>MLESKLKAPVFTATTQGDHYGEFVLEPLERGFGVTLGNPLRRILLSSIPGTAVTSVYIEDVLHEFSTIPGVKEDVVEIILNLKELVVRFLDPKMASTTLILRAEGPKEVRAGDFTPSADVEIMNPDLHIATLEEGGKLYMEVRVDRGVGYVPAERHGIKDRINAIPVDAIFSPVRRVAFQVEDTRLGQRTDLDKLTLRIWTDGSVTPLEALNQAVAILKEHLNYFANPEASLLPTPEVSKGEKRESAEEDLDLPLEELGLSTRVLHSLKEEGIESVRALLALNLKDLRNIPGIGERSLEEIRQALAKKGFTLKE[4x];>MEIKRFGRIREVIPLPPLTEIQVESYKKALQADVPPEKRENVGIQAAFKETFPIEEGDKGKGGLVLDFLEYRIGDPPFSQDECREKDLTYQAPLYARLQLIHKDTGLIKEDEVFLGHLPLMTEDGSFIINGADRVIVSQIHRSPGVYFTPDPARPGRYIASIIPLPKRGPWIDLEVEASGVVTMKVNKRKFPLVLLLRVLGYDQETLVRELSAYGDLVQGLLDEAVLAMRPEEAMVRLFTLLRPGDPPKKDKALAYLFGLLADPKRYDLGEAGRYKAEEKLGVGLSGRTLVRFEDGEFKDEVFLPTLRYLFALTAGVPGHEVDDIDHLGNRRIRTVGELMADQFRVGLARLARGVRERMVMGSPDTLTPAKLVNSRPLEAALREFFSRSQLSQFKDETNPLSSLRHKRRISALGPGGLTRERAGFDVRDVHRTHYGRICPVETPEGANIGLITSLAAYARVDALGFIRTPYRRVKNGVVTEEVVYMTASEEDRYTIAQANTPLEGDRIATDRVVARRRGEPVIVAPEEVEFMDVSPKQVFSLNTNLIPFLEHDDANRALMGSNMQTQAVPLIRAQAPVVMTGLEERVVRDSLAALYAEEDGEVVKVDGTRIAVRYEDGRLVEHPLRRYARSNQGTAFDQRPRVRVGQRVKKGDLLADGPASEEGFLALGQNVLVAIMPFDGYNFEDAIVISEELLKRDFYTSIHIERYEIEARDTKLGPERITRDIPHLSEAALRDLDEEGIVRIGAEVKPGDILVGRTSFKGEQEPSPEERLLRSIFGEKARDVKDTSLRVPPGEGGIVVGRLRLRRGDPGVELKPGVREVVRVFVAQKRKLQVGDKLANRHGNKGVVAKILPVEDMPHLPDGTPVDVILNPLGVPSRMNLGQILETHLGLAGYFLGQRYISPVFDGATEPEIKELLAEAFNLYFGKRQGEGFGVDKREKEVLARAEKLGLVSPGKSPEEQLKELFDLGKVVLYDGRTGEPFEGPIVVGQMFIMKLYHMVEDKMHARSTGPYSLITQQPLGGKAQFGGQRFGEMEVWALEAYGAAHTLQEMLTIKSDDIEGRNAAYQAIIKGEDVPEPSVPESFRVLVKELQALALDVQTLDEKDNPVDIFEGLASKR[2x];>[2x]MKKEVRKVRIALASPEKIRSWSYGEVEKPETINYRTLKPERDGLFDERIFGPIKDYECACGKYKRQRFEGKVCERCGVEVTRSIVRRYRMGHIELATPAAHIWFVKDVPSKIGTLLDLSATELEQVLYFNKYIVLDPKGAVLDGVPVEKRQLLTDEEYRELRYGKQETYPLPAGVDALVKDGEEVVKGQELAPGVVSRMDGVALYRFPRRVRVDYLRKERAALRIPLSAWVEKEAYRPGEVLAELSEPYLFRAEESGVVELKDLAEGHLIYLRQEEEVVARYFLPAGMTPLVVEGEIVEVGQPLAEGKGLLRLPRHMTAKEVEAEEEGDSVHLTLFLEWTEPKDYKVAPHMNVIVPEGAKVQAGEKIVAAIDPEEEVIAEAEGVVHLHEPASILVVKARVYPFEDDVEVTTGDRVAPGDVLADGGKVKSEIYGRVEVDLVRNVVRVVESYDIDARMGAEAIQELLKELDLEKLERELLEEMKHPSRARRAKARKRLEVVRAFLDSGNRPEWMILEAVPVLPPDLRPMVQVDGGRFATSDLNDLYRRLINRNNRLKKLLAQGAPEIIIRNEKRMLQEAVDAVIDNGRRGSPVTNPGSERPLRSLTDILSGKQGRFRQNLLGKRVDYSGRSVIVVGPQLKLHQCGLPKRMALELFKPFLLKKMEEKAFAPNVKAARRMLERQRDIKDEVWDALEEVIHGKVVLLNRAPTLHRLGIQAFQPVLVEGQSIQLHPLVCEAFNADFDGDQMAVHVPLSSFAQAEARIQMLSAHNLLSPASGEPLAKPSRDIILGLYYITQVRKEKKGAGMAFATPEEALAAYERGEVALNAPIVVAGRETSVGRLKFVFANPDEALLAVAHGLLDLQDVVTVRYLGRRLETSPGRILFARIVGEAVGDEKVAQELIQMDVPQEKNSLKDLVYQAFLRLGMEKTARLLDALKYYGFTLSTTSGITIGIDDAVIPEEKQRYLEEADRKLRQIEQAYEMGFLTDRERYDQVIQLWTETTEKVTQAVFKNFEENYPFNPLYVMAQSGARGNPQQIRQLCGMRGLMQKPSGETFEVPVRSSFREGLTVLEYFISSHGARKGGADTALRTADSGYLTRKLVDVAHEIVVREADCGTTNYISVPLFQMDEVTRTLRLRKRSDIESGLYGRVLAREVEALGRRLEEGRYLSLEDVHFLIKAAEAGEVREVPVRSPLTCQTRYGVCQKCYGYDLSMARPVSIGEAVGVVAAESIGEPGTQLTMRTFHTGGVAVGTDITQGLPRVIELFEARRPKAKAVISEIDGVVRIEEGEDRLSVFVESEGFSKEYKLPKDARLLVKDGDYVEAGQPLTRGAIDPHQLLEAKGPEAVERYLVDEIQKVYRAQGVKLHDKHIEIVVRQMLKYVEVTDPGDSRLLEGQVLEKWDVEALNERLIAEGKVPVAWKPLLMGVTKSALSTKSWLSAASFQNTTHVLTEAAIAGKKDELIGLKENVILGRLIPAGTGSDFVRFTQVVDQRTLKAIEEARKEAVEAKEKEAPRRPVRREQPGKGL;>[2x]MAEPGIDKLFGMVDSKYRLTVVVAKRAQQLLRHRFKNTVLEPEERPKMRTLEGLYDDPNAVTWAMKELLTGRLFFGENLVPEDRLQKEMERLYPTEEEA;>TSDPVRQYLHEIGQVPLLTLEEEIDLARKVEEGMEAIKKLSEATGLDQELIREVVRAKILGTARIQKIPGLKEKPDPKTVEEVDGKLKSLPKELKRYLHIAREGEAARQHLIEANLRLVVSIAKKYTGRGLSFLDLIQEGNQGLIRAVEKFEYKRRFKFSTYATWWIRQAINRAIADQARTIRIPVHMVETINKLSRTARQLQQELGREPSYEEIAEAMGPGWDAKRVEETLKIAQEPVSLETPIGDEKDSFYGDFIPDENLPSPVEAAAQSLLSEELEKALSKLSEREAMVLKLRKGLIDGREHTLEEVGAYFGVTRERIRQIENKALRKLKYHESRTRKLRDFLE[2x]

Transcription initiation is a major control point of gene expression. The initiation process is best understood in the bacterial system where the conserved ∼400 kD catalytic core of the RNA polymerase (RNAP or E, subunit composition α2ββ′ω) combines with the promoter-specificity factor σA to form the holoenzyme (EσA), which locates promoter DNA and unwinds 12–14 base pairs (bps) of the DNA duplex to yield the transcription-competent open promoter complex (RPo). Here, we determine crystal structures of Taq EσA bound to an us-fork promoter fragment, as well as a complete RPo, refined using diffraction data extending to 4.00 and 4.14 Å-resolution, respectively, allowing visualization of key features that stabilize the upstream edge of the transcription bubble. The results also reveal functionally relevant holoenzyme interactions with duplex DNA just upstream of the −10 element and potential protein/DNA interactions that direct the DNA template strand (t-strand) into the RNAP active site.

We therefore formed a complete RPo by combining Taq EΔ1.1σA with a duplex promoter DNA scaffold (−36 to +12 with respect to the transcription start site at +1) but with a non-complementary transcription bubble generated by altering the sequence of the t-strand DNA from −11 to +2. To stabilize the t-strand DNA, we added an RNA primer complementary to the ss t-strand DNA from +1 to −3, yielding a 4 bp RNA:DNA hybrid. We crystallized the resulting complex (437 kD, which we call RPo hereafter), collected and analyzed diffraction data, and refined the structure using reflections to a minimum Bragg spacing of 4.14 Å. In RPo, good electron density for all of the nucleic acids included in the scaffold was observed. The extensive protein/DNA interface in RPo buries 6300 Å2 of molecular surface. In the us-fork, the −11(t) nucleotide is absent, whereas in RPo, the −11(t) nucleotide is an (atypical) A, being part of the engineered non-complementary transcription bubble. In RPo, the A−11(t) base is not stacked on Y217 but instead is about 12 Å away, flipped up alongside the σ3A−3.0 α-helix, sitting between R288 and R291. At the point of melting, a ∼90° turn of the t-strand backbone (between −12 and −11) may be effected by electrostatic interactions between conserved basic residues of σ2A (R220) and σ3A (R288, R291) and four t-strand backbone phosphates in a row (−13, −12, −11, −10) encompassing the turn. Indeed, the upstream edge of the post-translocated 4-nt transcript fits snugly between the RNAP active site and the distal tip of the σ3.2-loop, which contacts the upstream RNA:DNA bp at −3, and the t-strand bases at −4 and −5.>MVHLNKTIQEGDNPDLTAERLTATFDTHAMAAQIYGGEMRARRRREITAKLAEIPELHDSMPLPYMTREEKIMESARKLTVLTQRMSEIIDPTDAGELYHLNNEVLGIEGNPMALHGVMFIPALNAQASDEQQAKWLIRALRREIIGTYAQTEMGHGTNLQNLETTATYDIGTQEFVLHTPKITALKWWPGNLGKSSNYAVVVAHMYIKGKNFGPHTFMVPLRDEKTHKPLPGITIGDIGPKMAYNIVDNGFLGFNNYRIPRTNLLMRHTKVEADGTYIKPPHAKINYSAMVHVRSYMLTGQAIMLSYALNIATRYSAVRRQGQIDKNEPEVKVLEYQTQQHRLFPFIARAYAFQFAGAETVKLYERVLKEMKSGNVSLMADLHALTSGLKSVVTHQTGEGIEQARMACGGHGYSMASYISEIYGVAIGGCTYEGENMVMLLQLARYLVKSAALVKSGKASQLGPLVAYLGARSEPTSLIDRVPNGGITEYIKTFQHIAKRQTLKAANKFFGLMENGEKREIAWNKSSVELNRASRLHTRLFIVEAFARRVNEIGDITIKEALSDLLHLHVNYELLDVATYALE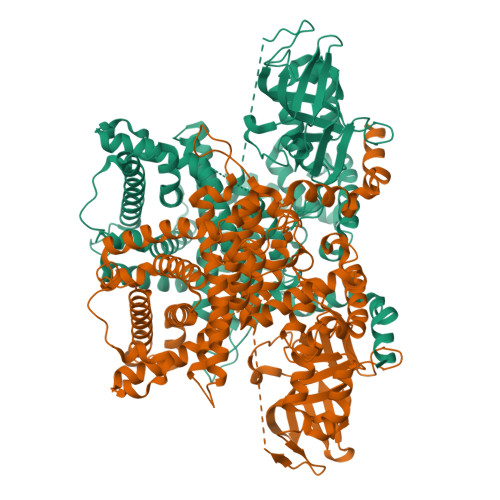DGFMSSTQLDYVRDQLYFYLQKIRPNAVSLLDSWEFSDRELRSVLGRRDGHVYENLFKWAKESPLNKTDVLPSVDTYLKPMMEKARQSKLHHHHHHHHHH[4x]> EKLGDISFSLRYVPTAGKLTVVILEAKNLKKMDVGGLSDPYVKI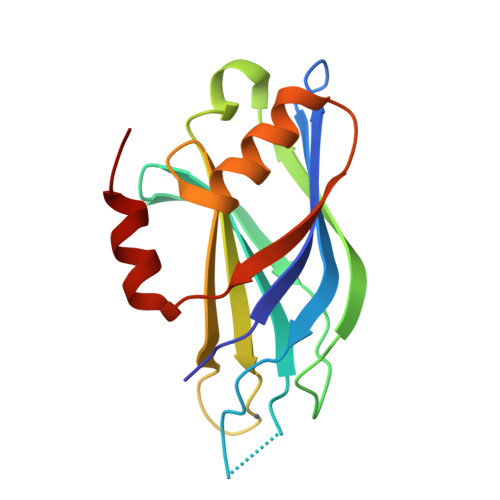HLMQNGKRLKKKKTTIKKNTLNPYYNESFSFEVPFEQIQKVQVVVTVLDYDKIGKNDAIGKVFVGYNSTGAELRHWSDMLANPRRPIAQWHTLQVEEEVDAMLAVKK(6R)-2-amino-6-methyl-5,6,7,8-tetrahydropteridin-4(3H)-one 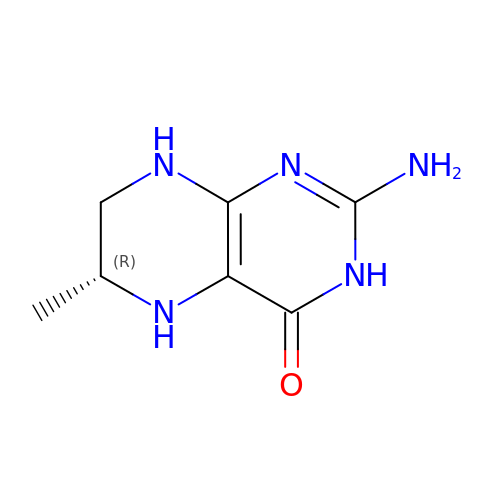| C7 H11 N5 O | HWOZEJJVUCALGB-GSVOUGTGSA-N>MADGEAAGQQADAVMPTGPAIDVLAFGDSLFAGYRLDRDESYPARLQAALRERGLNVNVTNAGVSGDTTAAGLQRIDFVLDSMAGEPDLVLLELGANDMLRGLPAEEARRNLDTILQRLDQRDIPVMVYGMRAAPNLGGDYGRSFDSIFPDLADKYDAELVP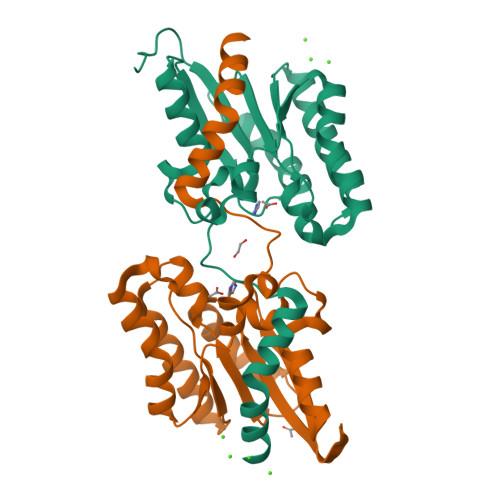FFIEPLIFDRSLVQQDQLHPTAQGVDAMVEQTVEQVEDRIDDL[2x]> GPLGSEVIQALIFKDDGSLGLSISGGVGSSSFKSGDDGIF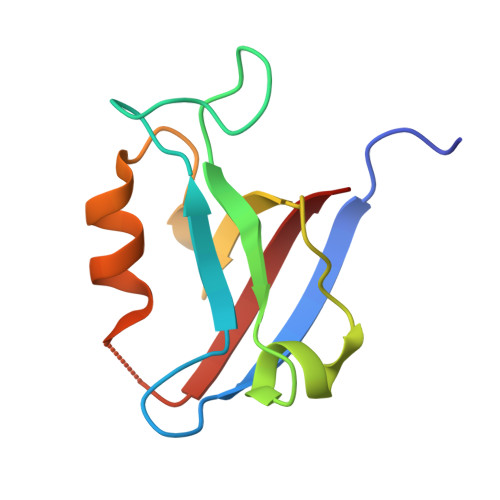VSKIAKGGPCDNEGTLKIGDKILSVNEISFTGITHEKAVEILKNQDSKYMVVVERS>MLSRSRCASRAFSRSLSAFQKGNCPLVRRSLPGISLCQGPGYPDSRKTVINSSNIFSVRFFRTTAVCKDDVITVKTPAFAESVTEGDVRWEKAVGDTVAEDEVVCEIETDKTSVQVPSPANGVIEALLVPDGGKVEGGTPLFTLRKTGAAPAKAKPAAAPAAAAPKAEPTVSAVPPPPAAPIPTQMPPVPSPSQPLTSKPVSAVKPTAAPPRAEAGAGVGLRSEHREKMNRMRQRIAQRLKEAQNTCAMLTTFNEIDMSNIQEMRARHKDAFLKKHNLKLGFMSAFVKASAFALQEQPVVNAVIDDATKEVVYRDYIDISVAVATPRGLVVPVIRNVETMNYADIERTISELGEKARKNELAIEDMDGGTFTISNGGVFGSLFGTPIINPPQSAILGMHAIVDRPVVIGGKVEVRP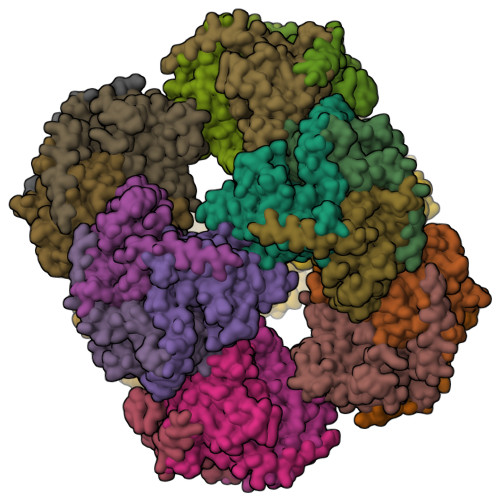MMYVALTYDHRLIDGREAVTFLRKIKAAVEDPRVLLLDL[24x]>MGIIRSILDTDLYKFTTGYAYAKLFPRAYGEFRFIDRNRQGFTEEFAELVRGEIRAMAALSLTRDEKEFLQRELPYLPPIYIDFLDGFRFDPEEVTVSIDAQGHLDIRAQGLLYRVTLWETPILAVISELYYRFIGAEPDWKQVEEVTRSKGELMREHRATFSIFGMRRRFSLEVEDRVTDILKQYAGESLFGTSNVHLAHKHGLRVSGTHPHEWIQFHGAIYGYKMANYVAMEDWINVYDGDLGTVLTDTYTTDVFMRNFSKKHAMLFTSLRHDSGDPEIFIEKAVRRYEELRVDPKIKYIIFSDSLTPQRAIEIQKLCAGRIKASFGIGTNLTNDVGGGVEPLNIVMKLWKCKMTAKDDWHYCVKLSDVDGKHTGEPEEI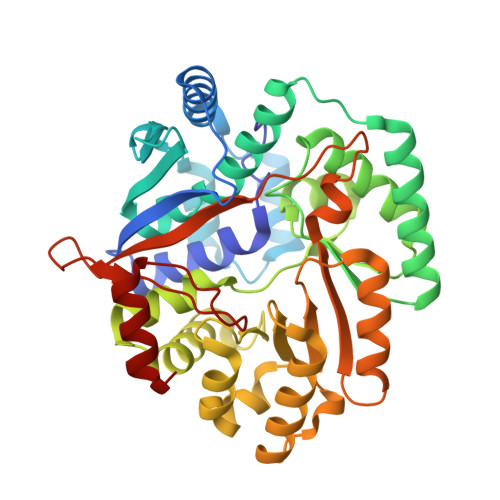LLAMNTLGIKPK[4x]>MHHHHHHMNVKKFPEGFLWGVATASYQIEGSPLADGAGMSIWHTFSHTPGNVKNGDTGDVACDHYNRWKEDIEIIEKLGVKAYRFSISWPRILPEGTGRVNQKGLDFYNRIIDTLLEKGITPFVTIFHWDLPFALQLKGGLLNREIADWFAEYSRVLFENFGDRVKNWITFNEPLCSAIPGYGSGTFAPGRQSTSEPWTVGHNILVAHGRAVKVFRETVKDGKIGIVLNGDFTYPWDAADPADKEAAERRLEFFTAWFADPIYLGDYPASMRKQLGDRLPTFTPEERALVHGSNDFYGMNHYTSNYIRHRSSPASADDTVGNVDVLFTNKQGNCIGPETAMPWLRPCAAGFRDFLVWISKRYGYPPIYVTENGAAFDDVVSEDGRVHDQNRIDYLKAYIGAMVTAVE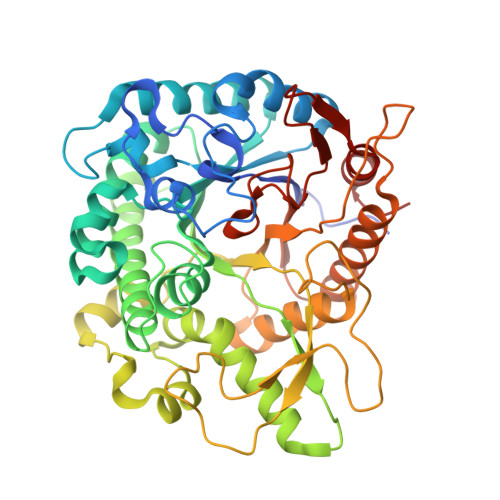LDGVNVKGYFVWSLLDNFEWAEGYSKRFGIVYVDYSTQKRIVKDSGYWYSNVVKNNGLED[3x]Far upstream element (FUSE) binding protein 1 (FUBP1 or FBP1) is a multifunctional single-stranded DNA- (ssDNA) and RNA-binding protein, which acts as a master regulator of diverse cellular processes including transcription, mRNA stability and translation as well as RNA splicing. Central to its single-stranded nucleic acid (ssNA) interacting function of human FUBP1 is a tandem of four K homology (KH) motifs, namely KH1, KH2, KH3 and KH4, which is embedded in the middle region in between the self-regulatory and transactivation domains at the N- and C- termini, respectively. Comparison of the four structures showed that they all adopted an evolutionarily conserved eukaryotic KH-domain architecture, consisting of a three-stranded β-sheet packed on one side by three helices. A common property in recognition of up to four nucleotides is facilitated by a ‘minimal KH motif’ that constructs an ssNA hydrophobic binding cleft formed on one side by two short consecutive helices (α1 and α2) and the GXXG-motif-containing connecting loop and on the other side by the domain’s β-sheet and the variable loop that links the β2 and β3.

In contrast to the upper part of the binding pocket, considerable variations of the amino acid compositions within α1 and the β2-β3 connecting loop led to the remarkably distinct properties of the nucleotide binding pocket at the lower half, which is responsible for interacting with ssDNA nucleobases. For instance, a longer loop together with the presence of small hydrophobic (A194 and A197) or polar residues (T385 and T388) in α1 of KH2 and 4, respectively, resulted in relatively open binding surface with strong positively-charged electrostatic potentials. In contrast, the migration patterns of KH2 and KH4 were rather ambiguous with some slight shifts observed for nearly all nucleotides, except fragment 4 and 10 that had a high GC-rich content. Interestingly, the potential interactions of KH2 and 4 with ssDNA 5–8, which shared the presence of a triple-repeated deoxythymidine (TTT), was consistent with the previous suggestion on the preference of FUBP1 for T-enriched sequence. In addition, we observed interestingly also that KH2 preferred the T-rich fragment 7 over the TGTG-core fragment 8, which was in contrast to KH4 that showed no preference for both ssDNA. As expected, in contrast to the wild type, all mutants did not show a shift in migration on native gels upon incubation with the selected ssDNA. These overall results suggested therefore that all four KH motifs of FUBP1 interacted with c-Myc FUSE ssDNA independently and individually, and KH1 and 3 might exert potential preference for ‘TTTGTGTT’ sequence while KH2 and KH4 might have broader binding specificity.

>SMNAVQEIMIPASKAGLVIGKGGETIKQLQERAGVKMVMIQDGPQNTGADKPLRITGDPYKVQQAKEMVLELIRDQG[4x]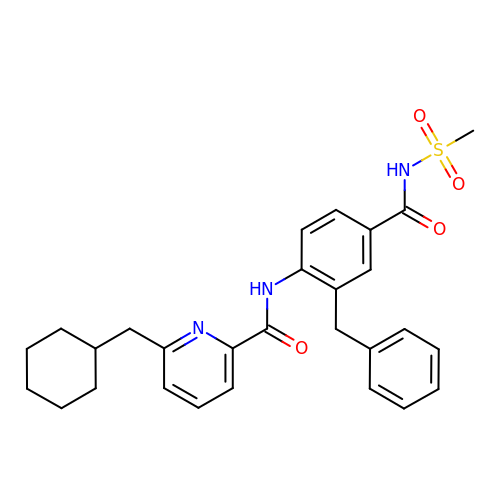6-(cyclohexylmethyl)-N-[4-(methylsulfonylcarbamoyl)-2-(phenylmethyl)phenyl]pyridine-2-carboxamide | C28 H31 N3 O4 S | ZNGZJFRXFZQBMG-UHFFFAOYSA-N> MRERPHTSGHHGAGEARATAPSTVSPYGPEARAELSSRLTTLRNTLAPATNDPRYLQACGGEKLNRFRDIQCRRQTAVRADLNANYIQVGNTRTIACQYPLQSQLESHFRMLAENRTPVLAVLASSSEIANQRFGMPDYFRQSGTYGSITVESKMTQQVGLGDGIMADMYTLTIREAGQKTISVPVVHVTTWPDFGVVSSEVTKALASLVDQTAE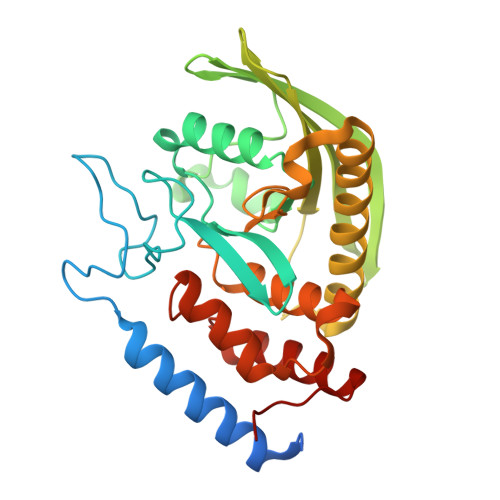TKRNMYESKGSSAVADDSKLRPVIHCRAGVGRTAQLIGAMCMNDSRNSQLSVEDMVSQMRVQRNGIMVQKDEQLDVLIKLAEGQGRPLLNS1,2,3,4-TETRAHYDROQUINOLIN-8-YL DIHYDROGEN PHOSPHATE | C9 H12 N O4 P | 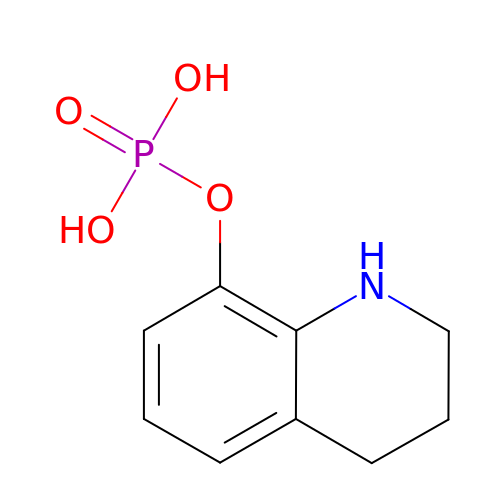NSJSAHCLJYVEDM-UHFFFAOYSA-N> EFYTAPSTESKFTEVLSKAKLQYPTSTTVAFADDLLDGYAASYFYLTSDLYMQFQVAGSSQRSELREMETSGDEAAWDCTGSTAHVASAQIAIPVQE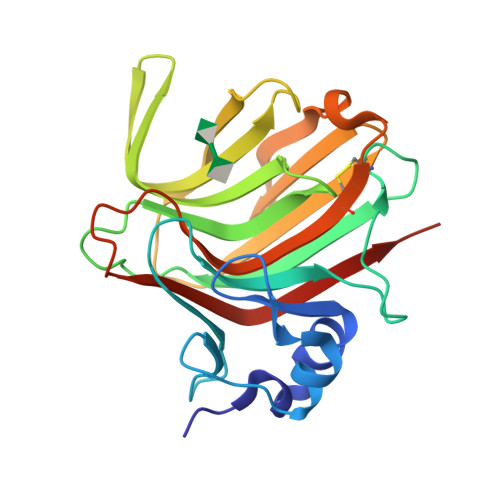DGIEEVTILQVHDSDVTPVLRISWVSSITIDGVTSEDVVLATIRNGIDDSTATKTVLQAHTTSRTEFNINVQNSKLSITVDGTTELDEADISQFDGSTCYFKAGAYNNNPTDTSANARIKMYELEWVDHHHHHH(1S)-4-[({3-hydroxy-2-methyl-5-[(phosphonooxy)methyl]pyridin-4-yl}methyl)amino]cyclopent-3-ene-1,3-dicarboxylic 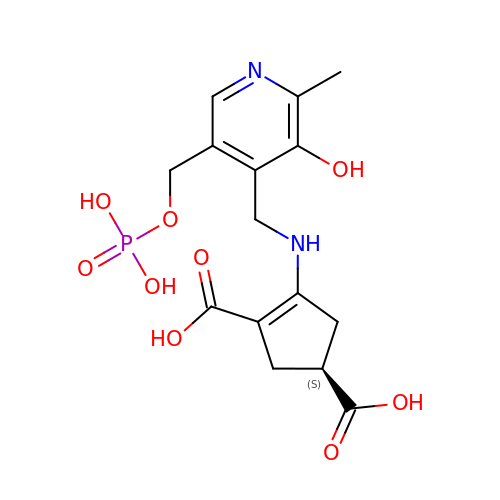acid | C15 H19 N2 O9 P | VNQKGJPXVHNUEY-QMMMGPOBSA-N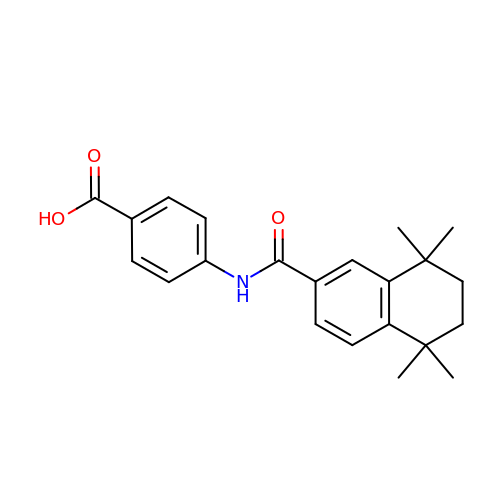4-{[(5,5,8,8-tetramethyl-5,6,7,8-tetrahydronaphthalen-2-yl)carbonyl]amino}benzoic acid | C22 H25 N O3 | SZWKGOZKRMMLAJ-UHFFFAOYSA-N> MGVVEEAHNVKVIGSGEATIVLGHGFGTDQSVWKHLVPHLVDDYRVVLYDNMGAGTTNPDYFDFDRYSNLEGYSFDLIAILEDLKIESCIFVGHSVSAMIGVLASLNRPDLFSKIVMISASPRYVNDVDYQGGFEQEDLNQLFEAIRSNYKAWCLGFAPLAVGGDMDSIAVQEFSRTLFNMRPDIALSVGQTIFQSDMRQILPFVTVPCHILQSVKDLAVPVVVSEYLHANLGCESVVEVIPSDGHLPQLSSPDSVIPVILRHIRNDIAMENLYFQ

Karrikin Insensitive 2 (KAI2) proteins are plant α/β-hydrolases with dual receptor-enzyme function that perceive smoke-derived karrikins (KARs) and an endogenous, yet undiscovered, KAI2 ligand (KL). Upon ligand binding, KAI2 is activated and interacts with its target proteins, including MAX2 and SMAX1, which initiate the physiological responses. KAI2 and D14 are α/β-hydrolases containing a Ser-His-Asp catalytic triad in their hydrophobic substrate-binding pockets, and therefore both proteins display hydrolytic activity toward various SL analogs, including GR24, desmethyl-GR24, and debranones compounds. Activation of KAI2 is thought to require hydrolysis of the ligand; however, this has not been experimentally proven.

6′-Carba-dMGer, in which the phenol ether oxygen of dMGer was replaced by a CH2 group, was also designed as a chemical tool that cannot form a covalent adduct with KAI2 because the butenolide ring does not dissociate from the biphenyl moiety. To elucidate the molecular interaction of KAI2 with the (+)-dMGer analogs, we analyzed the crystal structure of the KAI2–(+)-6′-carba-dMGer complex. We examined only the KAI2–(+)-6′-carba-dMGer complex because we were unable to crystallize the KAI2–(+)-dMGer and KAI2–(+)-1′-carba-dMGer complexes. The electron density map indicated that the KAI2-(+)-6′-carba-dMGer crystal structure was composed of two conformers: The ligand was bound in conformer A, whereas the ligand was not observed in conformer B. In conformer A, the butenolide ring of (+)-6′-carba-dMGer faced toward the bottom of the catalytic pocket, while the nitrobiphenyl moiety was oriented toward the access groove of the pocket and was partially exposed to the solvent. Additionally, the orientation of the side-chain phenyl ring of Phe26 in KAI2 was shifted in conformer A compared with apo-KAI2 and conformer B. The phenyl ring of Phe26 probably formed a π–π interaction with the phenyl ring of (+)-6′-carba-dMGer in conformer A. In conformer A, the butenolide ring of (+)-6′-carba-dMGer formed a strong hydrogen bond network with Phe26, Ser95, Tyr124, and His246 that was mediated by two water molecules. However, the O-1′ atom, not the 5′-carbonyl oxygen, was oriented toward the catalytic serine, probably because of the methylene group introduced instead of the phenol ether oxygen of (+)-dMGer. This orientation of the butenolide ring may prevent nucleophilic attack from the serine and explain the nonhydrolyzability of (+)-6′-carba-dMGer. In addition, analysis of the crystal structure of KAI2–(+)-6′-carba-dMGer indicated that (+)-6′-carba-dMGer bound to the catalytic pocket of KAI2 in an intact state.>MHLKIVCLSDEVREMYKNHKTHHEGDSGLDLFIVKDEVLKPKSTTFVKLGIKAIALQYKSNYYYKCEKSENKKKDDDKSNIVNTSFLLFPRSSISKTPLRLANSIGLIDAGYRGEIIAALDNTSDQEYHIK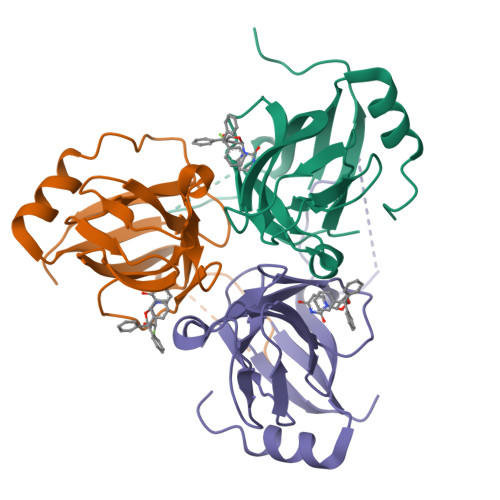KNDKLVQLVSFTGEPLSFELVEELDETSRGEGGFGSTSNNKY[3x]> SNAADPKTKGRGSGGNGSGRRLVIVESPTKARKLASYLGSGYIVESSRGHIRDLPRAASDVPAKYKSQPWARLGVNVDADFEPLYIISPEKRSTVSELRGLLKDVDELYLATDGDREGEAIAWHLLETLKPRIPVKRMVFHEITEPAIRAAAEHPRDLDIDLVDAQETRRILDRLYGYEVSPVLWKKVAPKLSAGRVQSVATRIIVARERDRMAFRSAAYWDILAKLDASVSDPDAAPPTFSARLTAVAGRRVATGRDFDSLGTLRKGDEVIVLDEGSATALAAGLDGTQLTVASAEEKPYARRPYPPFMTSTLQQEASRKLRFSAERTMSIAQ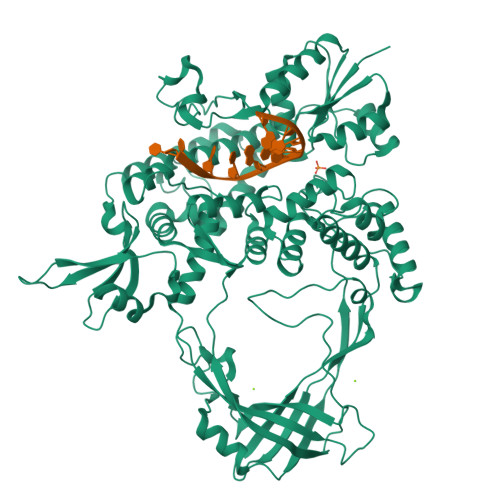RLYENGYITYMRTDSTTLSESAINAARTQARQLYGDEYVAPAPRQYTRKVKNAQEAHEAIRPAGETFATPDAVRRELDGPNIDDFRLYELIWQRTVASQMADARGMTLSLRITGMSGHQEVVFSATGRTLTFPGFLKAYVETVDELVGGEADDAERRLPHLTPGQRLDIVELTPDGHATNPPARYTEASLVKALEELGIGRPSTYSSIIKTIQDRGYVHKKGSALVPSWVAFAVTGLLEQHFGRLVDYDFTAAMEDELDEIAAGNERRTNWLNNFYFGGDHGVPDSVARSGGLKKLVGINLEGIDAREVNSIKLFDDTHGRPIYVRVGKNGPYLERLVAGDTGEPTPQRANLSDSITPDELTLQVAEELFAT> GPERTSIAVHALMG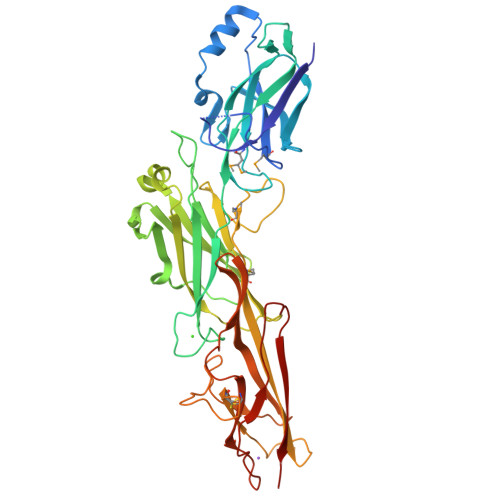LPTGQPANGTKLDSIGLPKVDGMSFTLYRVNEIDLTTQAGWDAASKIKLEELYTNGHPTDKVTKVATKKTEGGVAKFDNLTPALYLVVQELNGAEAVVRSQPFLVAAPQTNPTGDGWLQDVHVYPKHQALSEPVKTAVDPDATQPGFSVGENVKYRVATKIPEIASNTKFEGFTVADKLPAELGKPDTNKITVTLGGKPINSTDVSVQTYQVGDRTVLSVQLAGATLQSLDQHKDQELVVEFEAPVTKQPENGQLDNQAWVLPSNPTAQWDPEESGDAALRGMPSSRVSSKFGQITIEKSFDGNTPGADRTATFQLHRCEADGSLVKSDPPISLDGKQEFVTGQDGKAVLSGIHLGTLQLESNVMKYTDAWAGKGTEFCLVETATASGYELLPKPVIVKLEANESTNVLVEQKVKIDNKKKN>[2x]MAQSKGSVDQTLHAPHCEVGCAANVARRVGVDLARQVIGAHWASRMLVREVGTFPQPLLDRTQVTFSAQGEGWPALLARMTGGEVTSRHVPREELLSTLHADRAEGGTLLFMEDRACPWLDSAHSPGMLPHVVVPDGVAPDGSWQLIEGHSWWRGRYAMSEQDLLAASYPDPDPHHVAGRVLSLRIRPSAERAAQLDTLARQELAAGLRTYLA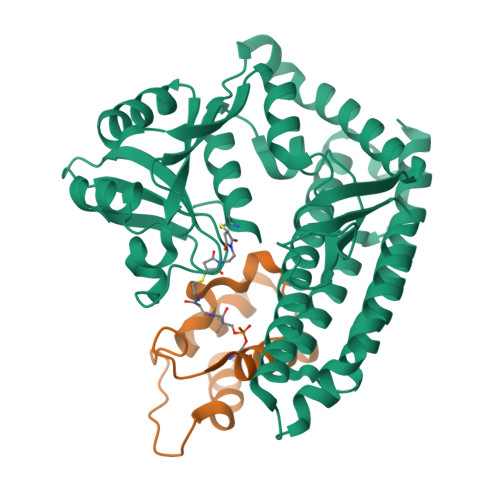AECGETETPAGRIVWANGPQSVPLLVERLRGWDYLCPLAARNDLSTEHARDVALGRYLFLALTDELAFAAYARAGTLRLVEGLGLAGAVGGLRPDEAWRLAWRSGQKLYRRLDRQNLSALFSALEKAAEVDVEYARRLLKELKLAAALEHHHHHHHH;>MSLLVDVLELLRPLLPSADTELTPDTELFSSQLLDSLALEEIQAAIESRWVPLPPEELTLANFNTPAAIAETIARTST[2x]> MKGFQFKVIQEKLQGRQFINSDKIKPDHPQTIIKKTLLKEYQSKNFSCQEERDLFLEFTEKIVQNFHNINFNYLLKKFCKLPENYQSLKSQVKQIVQSENKANQQSCENLFNSLYDTEISYKQITNFLRQIIQNCVPNQLLGKKNFKVFLEKLYEFVQMKRFENQKVLDYICFMDVFDVEWFVDLKNQKFTQKRKYISDKRKI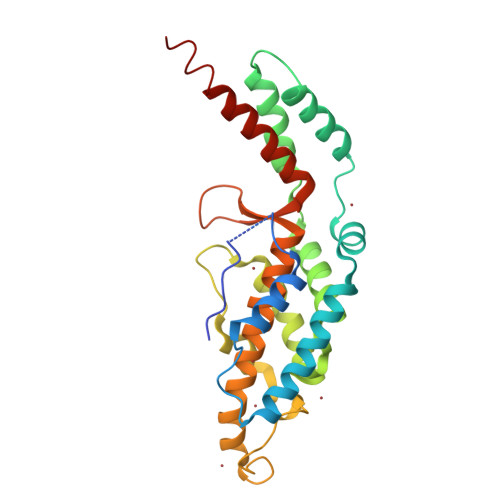LGDLIVFIINKIVIPVLRYNFYITEKHKEGSQIFYYRKPIWKLVSKLTIVKLEEENLEKVEEKL> GEIAALAVNAWKTTALKNAIAAAQKAGDAAGKIAGESKGVETIIGILEQYYSIYELKGTPLKSFFATTHYTDISNIATVIDTELNT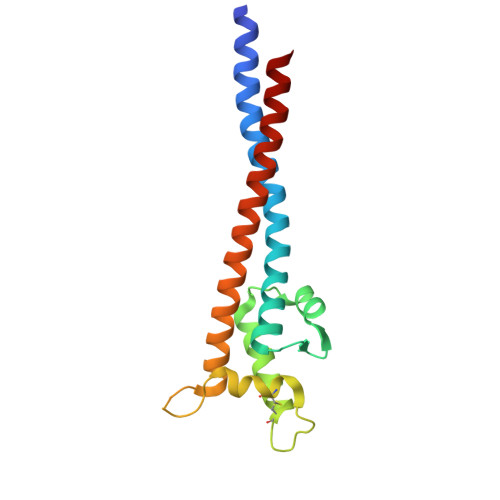SCGLNSLANQAICGLRTKLGLVAKPGQVMVTQKEAITKMITNVVHKSEITAEAAKTEVAATKTAAAIKMNTEAIEAA(dimethyl-lambda~4~-sulfanyl)acetic acid | C4 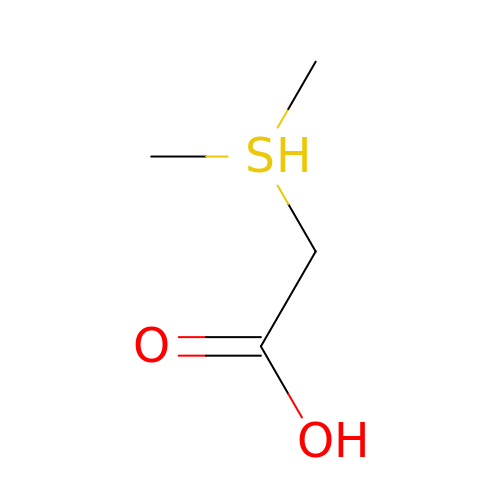H10 O2 S | GBHLSDCOGOHDJL-UHFFFAOYSA-N>MSR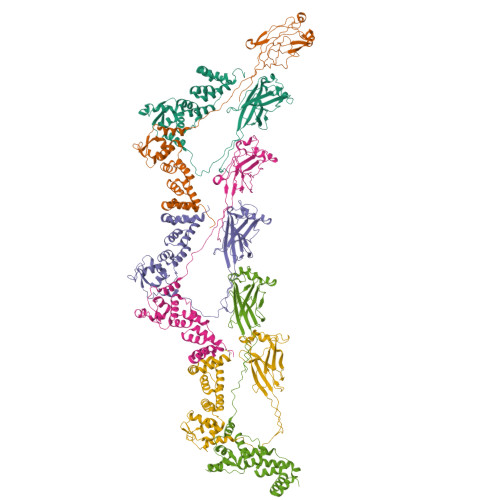VPSPPPPAEMSSGPVAESWCYTQIKVVKFSYMWTINNFSFCREEMGEVIKSSTFSSGANDKLKWCLRVNPKGLDEESKDYLSLYLLLVSCPKSEVRAKFKFSILNAKGEETKAMESQRAYRFVQGKDWGFKKFIRRDFLLDEANGLLPDDKLTLFCEVSVVQDSVNISGQNTMNMVKVPECRLADELGGLWENSRFTDCCLCVAGQEFQAHKAILAARSPVFSAMFEHEMEESKKNRVEINDVEPEVFKEMMCFIYTGKAPNLDKMADDLLAAADKYALERLKVMCEDALCSNLSVENAAEILILADLHSADQLKTQAVDFINYHASDVLETSGWKSMVVSHPHLVAEAYRSLASAQCPFLGPPRKRLKQ[6x]> GMASLKAKVLETFLAKSRPELLEYYIKVILDYNTAHNKVALSECYTVASVAEMPQNYRPHPQRFTYCSQVLGLHCYKKGIHYWEVELQKNNFCGVGICYGSMNRQGPESRLGRNSASWCVEWFNTKISAWHNNVEKTLPSTKATRVGVLLNCDHGFVIFFAVADKVHLMYKFRVDFTEALYPAFWVFSAGATLSICSPK

TRIM25 is a member of the TRIM family of RING-type E3 ligases and comprises a canonical N-terminal tripartite motif (TRIM) and a variable C-terminal PRYSPRY substrate binding domain. TRIM25 has been reported to ubiquitinate a number of different substrates, possibly in some cases mediated through RNA binding, including RIG-I,15,17,18 DDX3X19 and ZAP,20–22 with diverse roles in immune regulation, cancer signalling pathways and antiviral activity. We sought to assess whether the E3 ligase TRIM25, reported to catalyse the formation of both Lys48- and Lys63-linked ubiquitin chains, could be liganded and repurposed for targeted protein ubiquitination. As the majority of current proximity-inducing small molecules for E3s recruit substrates to the physiological substrate binding component (e.g. the substrate adaptor of Cullin RING E3s),11 we focused our efforts towards liganding the PRYSPRY substrate binding domain of TRIM25.

A crystal structure of the TRIM25 PRYSPRY-compound 10 complex was solved at 1.8 Å resolution, which, to our knowledge, represents the first published structure of TRIM25 in complex with a small molecule. Analysis by intact protein LCMS revealed Cys498 as the site of covalent modification by compound 10. Multiple sequence alignment of all PRYSPRY-containing TRIM proteins showed that Cys498 is not conserved across the family (ESI†). Thus, the covalent targeting of Cys498 by compound 10 reveals a unique binding mode for TRIM25. The biphenyl ring system of 10 forms π-stacking interactions with the aromatic side chains of Phe523, Phe554, Trp616, and Phe618. Furthermore, the carbonyl of the Cys-linked acetamide bond of 10 acts as an H-bond acceptor for both the side chain hydroxyl and main chain –NH of Ser499, and the side chain indole amine of Trp616. The carbonyl of the diazepane amide linker also forms an H-bond interaction with the terminal guanidino group of Arg541. Interestingly, structural overlay of TRIM25 PRYSPRY-compound 10 with the PRYSPRY domains of TRIM7, TRIM21 and TRIM58, for which small molecule ligands have been reported, showed that the ligands all bind at the same site on the PRYSPRY surface, which has also been suggested to be a substrate binding interface (ESI†). The meta position on the pendant phenyl ring was determined to be both solvent accessible and synthetically tractable. Interestingly, the rate of TRIM25 auto-ubiquitination was significantly increased by compounds 10 and 11 (ESI†).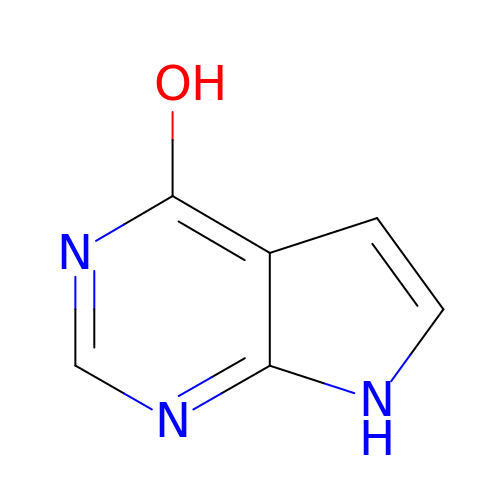7H-pyrrolo[2,3-d]pyrimidin-4-ol | C6 H5 N3 O | FBMZEITWVNHWJW-UHFFFAOYSA-N> ETGAKNLEPVSWSSLNPKFLSGKGLVIYPKIGDKLDIICPRAEAGRPYEYYKLYLVRPEQAAACSTVLDPNVLVTCNRPEQEIRFTIKFQEFSPNYMGLEFKKHHDYYITSTSNGSLEGLENREGGVCRTRTMKIIMKVGQDGT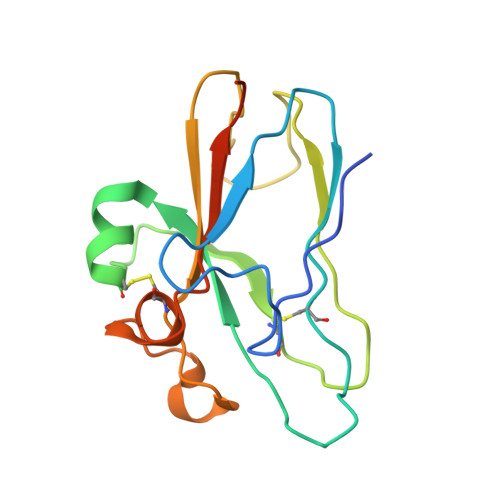KHHHHHH>[2x]MGHMMSNAEAFYASIRTELESIRAAGLFKNERVIATPQGARVRTTDGREVINLCANNYLGLSSHPQVIEAAHEALRTHGFGLSSVRFICGTQDLHKTLEARLSAFLGTEDTILYGSAFDANGGLFETLLGAEDAVISDALNHASIIDG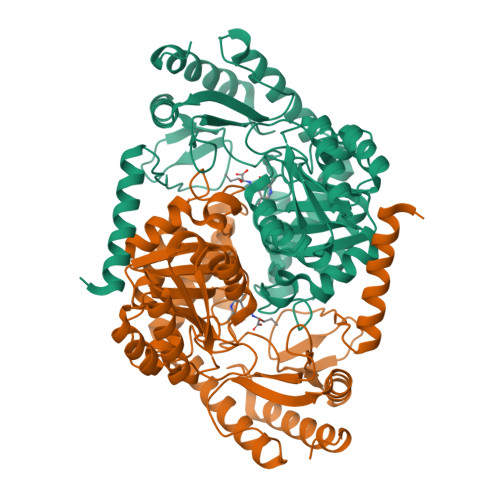VRLSKARRYRYQHNDMDDLRVQLEQARADGARYTLVFSDGVFSMDGTVARLDEMRAICDEYGALLGIDECHATGFMGQRGRGTHEARGVFGKIDIITGTLGAALGGASGGFTSARKEVVALLRQRSRPYLFSNTVAPAIVGASIAVLDILEASTELRDRLEGNTRFFRAGLDRLGFDVKAGDHPIIPIMVYDADKAQQLAQRLLELGVYVVGFFYPVVPKGQARIRVQMSALHDEAALQAALDAFGQAGRELGLILEHHHHHH(4~{E})-2-(3,4-dimethylphenyl)-4-[(1-methylpyrazol-4-yl)methylidene]-1,3-oxazol-5-one | C16 H15 N3 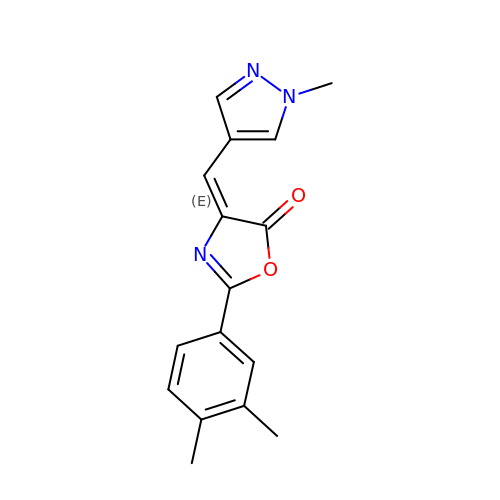O2 | BNKZAUBGRRNYQS-VGOFMYFVSA-N>MGNNTSSSEKADDNSYYVGGHKKSTDVPWYLEGDDEYELLLDVKGNIKGGSKEALVSHLTHHLSLDSNFNAVFLLMFSSMMSLGELISLLIARFNIEPPEGLSYEEYNLWVSKKRNPIRLRVINIMKLLLEKNWSMSYYNEPVLRRWLTFAHSDQVQTYSLGNLLVNYLERLLRGERIYVE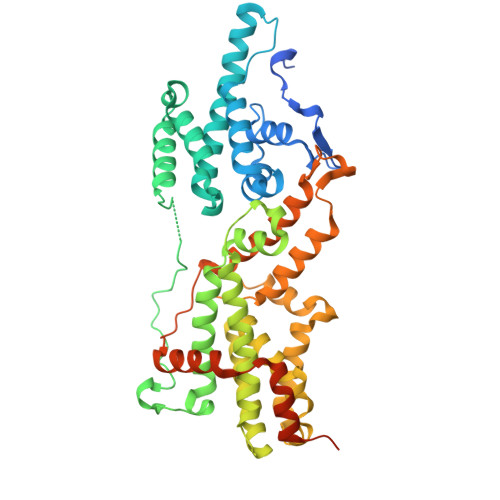RDPVIPNTKPPAPLTKGSSLSKKPRVMDIDYVELARQLTLREFKLYCKITKFACLAKVWGKKSGLSESIDSITQFIKASNQLTNFVGYMILRKADPKKRVQIIRYFIQVADKCRQYNNFSSMTAIISALYSSPIHRLKKTWEYMNADALSNLKNMNKLMNSSRNFNEYRDVLKFIGSEPCVPFFGVYLSDLTFVYHGNPDYLYNRTRQVNFAKRAKTSEIVSGIDRFKTTGYNFQEVPEIQKFLDAWFEKCPTIDEQYQISLNLEPREQPAGASNSNSTTNATTNIKSFKPFSLK[2x]> MSFTNATFSQVLDDLSARFILNLPAEEQSSVERLCFQIEQAHWFYEDFIRAQNDQLPSLGLRVFSAKLFAHCPLLWKWSKVHEEAFDDFLRYKTRIPVRGAIMLDMSMQQCVLVKGWKASSGWGFPKGKIDKDESDVDCAIREVYEETGFDCSSRINPNEFIDMT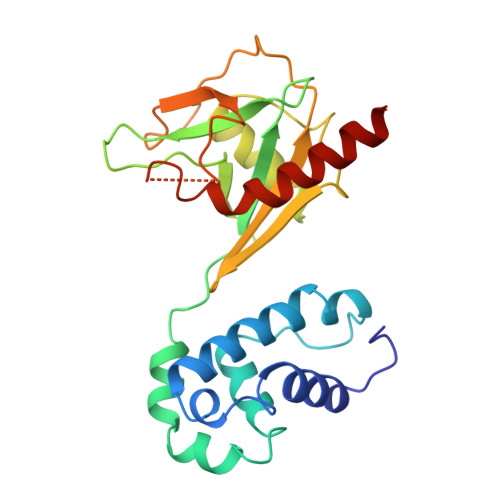IRGQNVRLYIIPGISLDTRFESRTRKEISKIEWHNLMDLPTFKKNKPQTMKNKFYMVIPFLAPLKKWIKKRNIANNT> MSQPRTPEQALDTPGDCPPGRRDEDAGEGIQCSQRMLSFSDALLSIIATVMILPVTHTEISPEQQFDRSVQRLLATRIAVYLMTFLIVTVAWAAHTRLFQVVGKTDDTLALLNLACMMTITFLPYTFSLMVTFPDVPLGIFLFCVCVIAIGVVQALIVGYAFHFPHLLSPQIQRSAHRALYRRHVLGIV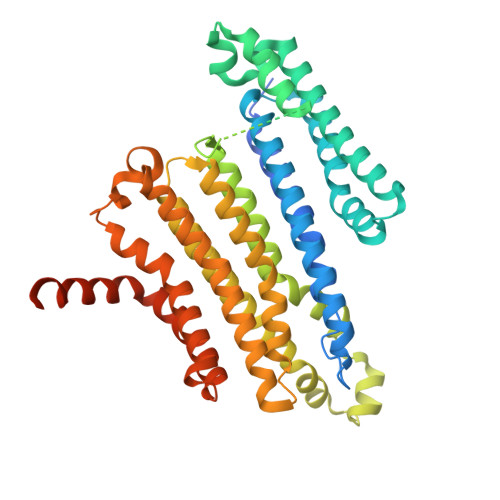LQGPALCFAAAIFSLFFVPLSYLLMVTVILLPYVSKVTGWCRDRLLGHREPSAHPVEVFSFDLHEPLSKERVEAFSDGVYAIVATLLILDICEDNVPDPKDVKERFSGSLVAALSATGPRFLAYFGSFATVGLLWFAHHSLFLHVRKATRAMGLLNTLSLAFVGGLPLAYQQTSAFARQPRDELERVRVSCTIIFLASIFQLAMWTTALLHQAETLQPSVWFGGREHVLMFAKLALYPCASLLAFASTCLLSRFSVGIFHLMQIAVPCAFLLLRLLVGLALATLRVLRGLARPEHPPPAPTGQDDPQSQLLPAPC>[4x]MEQRASLDSEESESPPQENSCLDPPDRDPNCKPPPVKPHIFTTRSRTRLFGKGDSEEASPLDCPYEEGGLASCPIITVSSVLTIQRPGDGPASVRPSSQDSVSAGEKPPRLYDRRSIFDAVAQSNCQELESLLPFLQRSKKRLTDSEFKDPETGKTCLLKAMLNLHNGQNDTIALLLDVARKTDSLKQFVNASYTDSYYKGQTALHIAIERRNMTLVTLLVENGADVQAAANGDFFKKTKGRPGFYFGELPLSLAACTNQLAIVKFLLQNSWQPADISARDSVGNTVLHALVEVADNTVDNTKFVTSMYNEILILGAKLHPTLKLEEITNRKGLTPLALAASSGKIGVLAY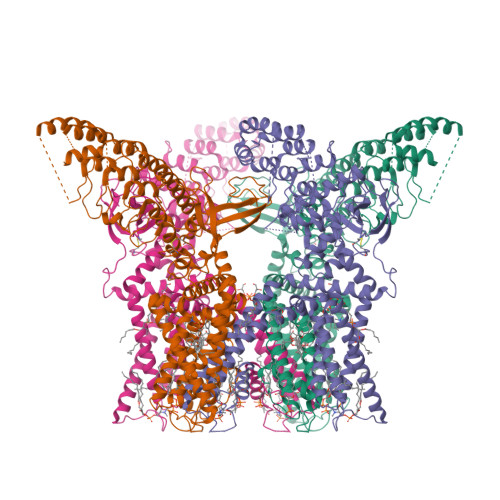ILQREIHEPECRHLSRKFTEWAYGPVHSSLYDLSCIDTCEKNSVLEVIAYSSSETPNRHDMLLVEPLNRLLQDKWDRFVKRIFYFNFFVYCLYMIIFTAAAYYRPVEGLPPYKLKNTVGDYFRVTGEILSVSGGVYFFFRGIQYFLQRRPSLKSLFVDSYSEILFFVQSLFMLVSVVLYFSQRKEYVASMVFSLAMGWTNMLYYTRGFQQMGIYAVMIEKMILRDLCRFMFVYLVFLFGFSTAVVTLIEDGKNNSLPMESTPHKCRGSACKPGNSYNSLYSTCLELFKFTIGMGDLEFTENYDFKAVFIILLLAYVILTYILLLNMLIALMGETVNKIAQESKNIWKLQRAITILDTEKSFLKCMRKAFRSGKLLQVGFTPDGKDDYRWCFRVDEVNWTTWNTNVGIINEDPGNCEGVKRTLSFSLRSGRVSGRNWKNFALVPLLRDASTRDRHATQQEEVQLKHYTGSLKPEDAEVFKDSMVPGEKENSLEVLFQGPDYKDDDDKAHHHHHHHHHH>[16x]MAPTWFYNTTNSEKLRELQHVLGGSAKLGYLTAKVTEILDVDLETV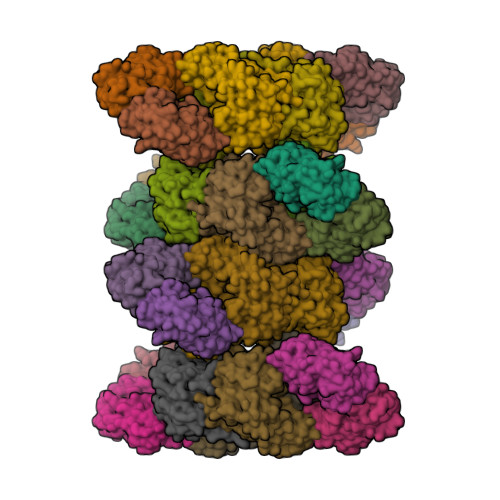IRAKAIAAYRAVRVPVIVEHGALCIDALNGLPGALVKPFWESLDTRLCEVIPAGQRTARARGALCYCDGRERHVLIEETEGEIAPSARGTGGFHWDPIFIPKGQTRTFAEMSLDEKLSFSPLGRLHTRLRTELGL;>MTTLTLSEAAPLLKKEFREGRLIPFLGAGFSKPLKLPDGSQLIASLAKTLGFEPELFDMHGRFEQLAEFFAISAPNRLQRLVYEMSLSFDSAEAEALREKSPMHRALAALDWRTIYTTNYDKHVEGALRDAGKQAAVLASFADFQGPRARDVCEVIKFHGTLDQPDTIVLTESSYFQRMALDAPPDQRLRADLLANSFLFIGYSFSDTNIRYIWYRMNQLREQSQLGVKHSQARRCFFATHGAGLVQPDILQQWNIDVIQLDPTDKSASVARLLESIA[16x]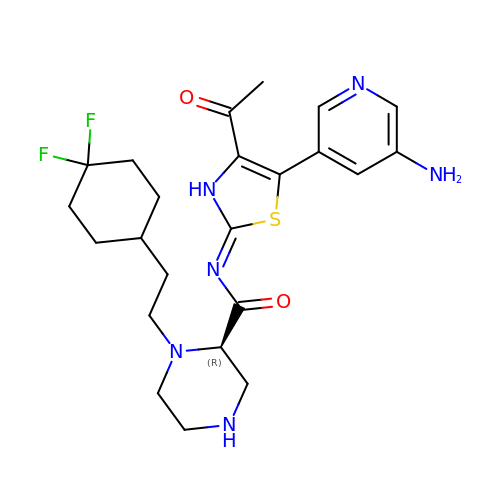(~{N}~{Z},2~{R})-~{N}-[5-(5-azanylpyridin-3-yl)-4-ethanoyl-3~{H}-1,3-thiazol-2-ylidene]-1-[2-[4,4-bis(fluoranyl)cyclohexyl]ethyl]piperazine-2-carboxamide | C23 H30 F2 N6 O2 S | OVBCFTIQGNIZAI-GOSISDBHSA-N> SMAGMSQRPPSMYWCVGPEESAVCPERAMETLNGAGDTGGKPSTRGGDPAARSRRTEGIRAAYRRGDRGGARDLLEEACDQCASQLEKGQLLSIPAAYGDLEMVRYLLSKRLVELPTEPTDDNPAVVAAYFGHTAVVQELLESLPGPCSPQRLLNWMLALACQRGHLGVVKLLVLTHGADPESYAVRKNEFPVIVRLPLYAAIKSGNEDIAIFLLRHGAYFCSYILLDSPDPSKHLLRKYFIEASPLPSSYPGKTALRVKWSHLRLPWVDLDWLIDISCQITELDLSANCLATLPSVIPWGLINLRKLNLSDNHLGELPGVQSSDEIICSRLLEIDISSNKLSHLPPGFLHLSKLQKLTASKNCLEKLFEEENATNWIGLRKLQELDISDNKLTELPALFLHSFKSLNSLNVSRNNLKVFPDPWACPLKCCKASRNALECLPDKMAVFWKNHLKDVDFSENALKEVPLGLFQLDALMFLRLQGNQLAALPPQEKWTCRQLKTLDLSRNQLGKNEDGLKTKRIAFFTTRGRQRSGTEAASVLEFPAFLSESLEVLCLNDNHLDTVPPSVCLLKSLSELYLGNNPGLRELPPELGQLGNLWQLDTEDLTISNVPAEIQKEGPKAMLSYLRAQLRKAEKCKLMKMIIVGPPRQGKSTLLEILQTGRAPQVVHGEATIRTTKWELQRPAGSRAKVESVEFNVWDIGGPASMATVNQCFFTDKALYVVVWNLALGEEAVANLQFWLLNIEAKAPNAVVLVVGTHLDLIEAKFRVERIATLRAYVLALCRSPSGSRATGFPDITFKHLHEISCKSLEGQEGLRQLIFHVTCSMKDVGSTIGCQRLAGRLIPRSYLSLQEAVLAEQQRRSRDDDVQYLTDRQLEQLVEQTPDNDIKDYEDLQSAISFLIETGTLLHFPDTSHGLRNLYFLDPIWLSECLQRIFNIKGSRSVAKNGVIRAEDLRMLLVGTGFTQQTEEQYFQFLAKFEIALPVANDSYLLPHLLPSKPGLDTHGMRHPTANTIQRVFKMSFVPVGFWQRFIARMLISLAEMDLQLFENKKNTKSRNRKVTIYSFTGNQRNRCSTFRVKRNQTIYWQEGLLVTFDGGYLSVESSDVNWKKKKSGGMKIVCQSEVRDFSAMAFITDHVNSLIDQWFPALTATESDGTPLMEQYVPCPVCETAWAQHTDPSEKSEDVQYFDMEDCVLTAIERDFISCPRHPDLPVPLQELVPELFMTDFPARLFLENSKLEHSEDEGSVLGQGGSGTVIYRARYQGQPVAVKRFHIKKFKNFANVPADTMLRHLRATDAMKNFSEFRQEASMLHALQHPCIVALIGISIHPLCFALELAPLSSLNTVLSENARDSSFIPLGHMLTQKIAYQIASGLAYLHKKNIIFCDLKSDNILVWSLDVKEHINIKLSDYGISRQSFHEGALGVEGTPGYQAPEIRPRIVYDEKVDMFSYGMVLYELLSGQRPALGHHQLQIAKKLSKGIRPVLGQPEEVQFRRLQALMMECWDTKPEKRPLALSVVSQMKDPTFATFMYELCCGKQTAFFSSQGQEYTVVFWDGKEESRNYTVVNTEKGLMEVQRMCCPGMKVSCQLQVQRSLWTATEDQKIYIYTLKGMCPLNTPQQALDTPAVVTCFLAVPVIKKNSYLVLAGLADGLVAVFPVVRGTPKDSCSYLCSHTANRSKFSIADEDARQNPYPVKAMEVVNSGSEVWYSNGPGLLVIDCASLEICRRLEPYMAPSMVTSVVCSSEGRGEEVVWCLDDKANSLVMYHSTTYQLCARYFCGVPSPLRDMFPVRPLDTEPPAASHTANPKVPEGDSIADVSIMYSEELGTQILIHQESLTDYCSMSSYSSSPPRQAARSPSSLPSSPASSSSVPFSTDCEDSDMLHTPGAASDRSEHDLTPMDGETFSQHLQAVKILAVRDLIWVPRRGGDVIVIGLEKDSGAQRGRVIAVLKARELTPHGVLVDAAVVAKDTVVCTFENENTEWCLAVWRGWGAREFDIFYQSYEELGRLEACTRKRR

Leucine Rich Repeat Kinase 1 and 2 (LRRK1 and LRRK2) are homologs in the ROCO family of proteins in humans. LRRK1 and LRRK2 have a similar domain organization: an N-terminal half containing Ankyrin (ANK) and Leucine Rich Repeats (LRR), and a catalytic C-terminal half containing the ROC–COR ROCO signature, followed by the kinase and a WD40 domain. Despite their shared domain architecture and involvement in intracellular trafficking, their disease associations are strikingly different: LRRK2 is involved in familial Parkinson’s disease while LRRK1 is linked to bone diseases. LRRK1 and LRRK2 use different mechanisms of autoinhibition, with LRRK1 having a second level of autoinhibition absent in LRRK2.

Our initial model for the kinase domain of LRRK1 showed density in the back pocket of the kinase that was not accounted for by the model. The density was located where Y1410 from the DYG motif would dock in the DYG ‘in’, or active, conformation. Symmetry expansion and focused refinement of the dimer dataset showed that a loop from the COR-B domain (residues 1,048–1,082), which is predicted by AlphaFold to be entirely disordered, threads into the kinase domain active site. The side chain of F1065, at the tip of the loop, sits inside the back pocket of the kinase, occupying the position of Y1410 in the DYG-in conformation. A similar ‘plugging’ of the kinase back pocket was observed in the DDR1 kinase. This suggests that the COR-B loop is an autoinhibitory element in LRRK1. We tested this by measuring Rab7a phosphorylation in 293T cells expressing either WT LRRK1 or LRRK1(F1065A), which we expected would at least partially relieve the autoinhibition. In agreement with this, the F1065A mutation led to a two-fold increase in the level of Rab7a phosphorylation in cells, comparable to that observed with the hyperactive K746G mutant. Our structure provides a mechanistic explanation for this activation: phosphorylation of these residues disrupts the loop, which is nestled against the kinase domain, releasing F1065 from the kinase’s back pocket and allowing the DYG motif to adopt the active ‘in’ conformation. The autoinhibitory COR-B loop is unique to LRRK1 and provides an additional level of regulation, present in both our monomer and dimer structures.>NAESSNPPQKMAFKAFGSPKKEKKESLSDFS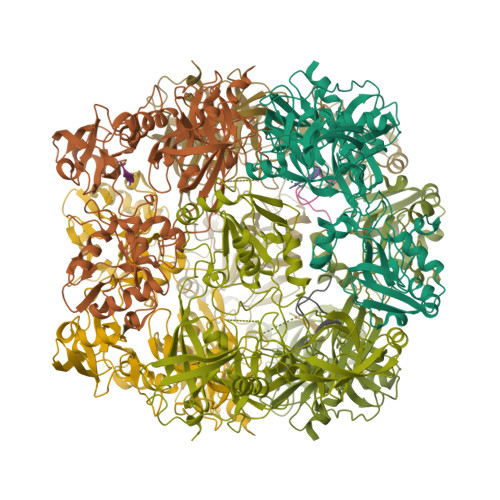RDQQTDPAKIHDASFLNAVVKVYCTHTAPDYSLPWQKQRQFTSTGSAFMIGDGKLLTNAHCVEHDTQVKVKRRGDDRKYVAKVLVRGVDCDIALLSVESEDFWKGAEPLRLGHLPRLQDSVTVVGYPLGGDTISVTKGVVSRIEVTSYAHGSSDLLGIQIDAAINPGNSGGPAFNDQGECIGVAFQVYRSEETENIGYVIPTTVVSHFLTDYERNGKYTGYPCLGVLLQKLENPALRECLKVPTNEGVLVRRVEPTSDASKVLKEGDVIVSFDDLHVGCEGTVPFRSSERIAFRYLISQKFAGDIAEIGIIRAGEHKKVQVVLRPRVHLVPYHIDGGQPSYIIVAGLVFTPLSEPLIEEECEDTIGLKLLTKARYSVARFRGEQIVILSQVLANEVNIGYEDMNNQQVLKFNGIPIRNIHHLAHLIDMCKDKYLVFEFEDNYVAVLEREASNSASLCILKDYGIPSERSADLLEPYVDPIDDTQALDQGIGDSPVSNLEIGFDGLVWA[3x]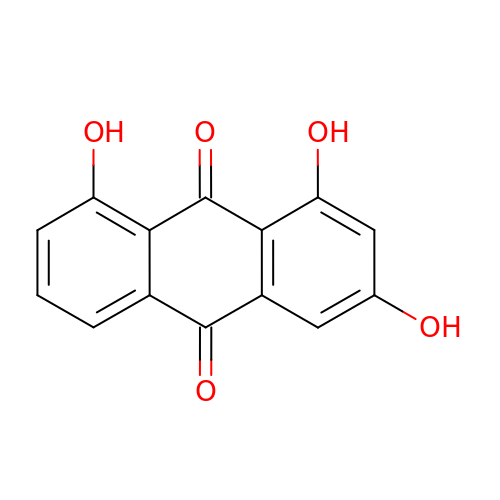1,3,8-tris(oxidanyl)anthracene-9,10-dione | C14 H8 O5 | VVEKCQAFOLKNKB-UHFFFAOYSA-N> ASPELASGKVWIRYPI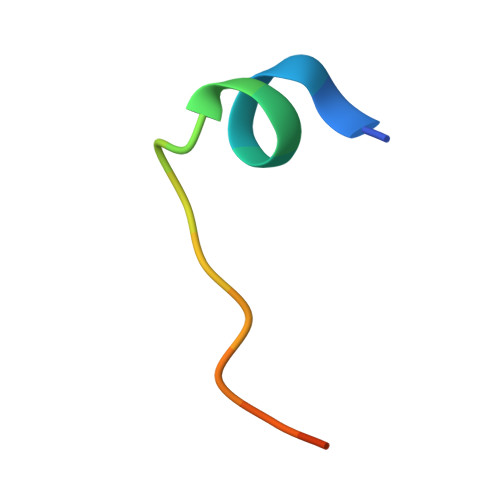VR> MEGSTGFDGDATTFFAPDAVFGDRVRRFQEFLDTFTSYRDSVRSIQVYNSNNAANYNDDQDDADERDLLGDDDGDDLEKEKKAASSTSLNILPHRIIISLDDLREFDRSFWSGILVEPAYFIPPAEKALTDLADSMDDVPHPNASAVSSRHPWKLSFKGSFGAHALSPRTLTAQHLNKLVSVEGIVTKTSLVRPKLIRSVHYAAKTGRFHYRDYTDATTTLTTRIPTPAIYPTEDTEGNKLTTEYGYSTFIDHQRITVQEMPEMAPAGQLPRSIDVILDDDLVDKTKPGDRVNVVGVFKSLGAGGMNQSNSNTLIGFKTLILGNTVYPLHARSTGVAARQMLTDFDIRNINKLSKKKDIFDILSQSLAPSIYGHDHIKKAILLMLMGGVEKNLENGSHLRGDINILMVGDPSTAKSQLLRFVLNTASLAIATTGRGSSGVGLTAAVTTDRETGERRLEAGAMVLADRGVVCIDEFDKMTDVDRVAIHEVMEQQTVTIAKAGIHTTLNARCSVIAAANPVFGQYDVNRDPHQNIALPDSLLSRFDLLFVVTDDINEIRDRSISEHVLRTHRYLPPGYLEGEPVRERLNLSLAVGEDADI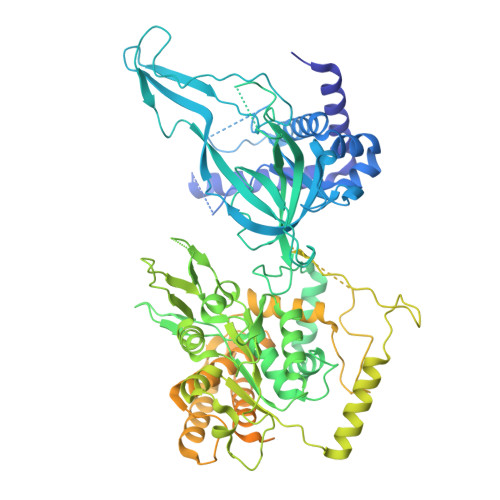NPEEHSNSGAGVENEGEDDEDHVFEKFNPLLQAGAKLAKNKGNYNGTEIPKLVTIPFLRKYVQYAKERVIPQLTQEAINVIVKNYTDLRNDDNTKKSPITARTLETLIRLATAHAKVRLSKTVNKVDAKVAANLLRFALLGEDIGNDIDEEESEYEEALSKRSPQKSPKKRQRVRQPASNSGSPIKSTPRRSTASSVNATPSSARRILRFQDDEQNAGEDDNDIMSPLPADEEAELQRRLQLGLRVSPRRREHLHAPEEGSSGPLTEVGTPRLPNVSSAGQDDEQQQSVISFDNVEPGTISTGRLSLISGIIARLMQTEIFEEESYPVASLFERINEELPEEEKFSAQEYLAGLKIMSDRNNLMVADDKVWRV> AVVASLKPLGFIASAIADGVTDTQVLLPDGASEHDYSLRPSDVKRLQGADLVVWVGPEMEAFMEKSVRNIPDN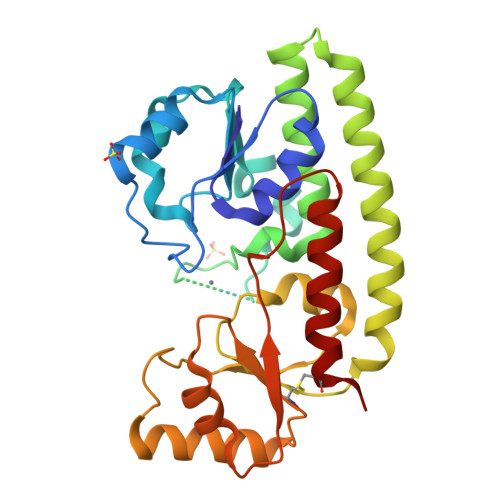KQVTIAQLADVKPLLMKGADDDEDEHAHTGADEEKGDVHHHHGEYNMHLWLSPEIARATAVAIHEKLVELMPQSRAKLDANLKDFEAQLAATDKQVGNELAPLKGKGYFVFHDAYGYYEKHYGLTPLGHFTVNPEIQPGAQRLHEIRTQLVEQKATCVFAEPQFRPAVVEAVARGTSVRMGTLDPLGTNIKLGKTSYSAFLSQLANQYASCLKGD> DFQSESYKDAYSRINAIVIEGEQEAFDNYNRLAEMLPDQRDELHKLAKMEQRHMKGFMACGKNLSVTPDMGFAQKYYERLHENFKAAAAEGKVVTCLLIQSLIIECFAIAAYN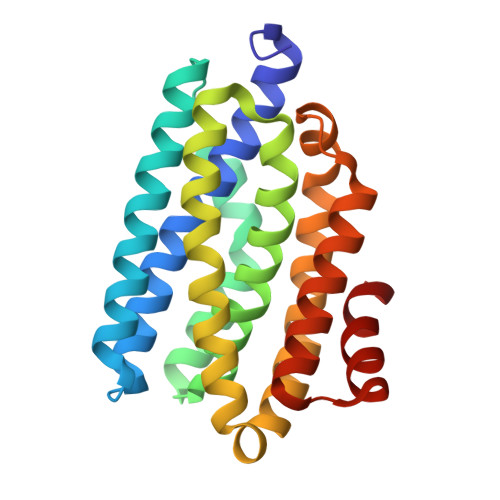IYIPVADAFARKITEGVVRDEYLHRNFGEEWLKANFDASKAELEEANRQNLPLVWLMLNEVADDARELGMERESLVEDFMIAYGEALENIGFTTREIMRMSAYGLAA>GSHMLEGGVEVLSVVTGEDSITQIELYLNPRMGVNSPDLPTTSNWYTYTYDLQPKGSSPDQPIKENLPAYSVARVSLPMLNEDITCDTLQMWEAISVKTEVVGISSLINVHYWDMKRVHDYGAGIPVSGVNYHMFAIGGEPLDLQGLVLDYQTQYPKTTNGGPITIETVLGRKMTPKNQGLDPQAKAKLDKDGNYPIEVWCPDPSKNENSRYYGSIQTGSQTPTVLQFSNTLTTVLLDENGVGPLCKGDGLFISCADIVGFLFKTSGKMALHGLPRYFNVTLRKRWVKN[20x]

The human Merkel cell polyomavirus (MCPyV or MCV) was discovered in 2008 and found to be clonally integrated into Merkel cell carcinomas (MCCs), establishing it as the first human oncovirus from the polyomavirus family. Polyomavirus infectious entry is initiated by the major capsid protein VP1, which attaches to cellular receptors to promote internalization and transport of the viral genome into the nucleus for replication. MCPyV VP1 is a symmetric ring-shaped homopentamer with the five VP1 monomers arranged around a central five-fold axis. Each monomer is composed of two antiparallel β-sheets, which together form a β-sandwich with jelly-roll topology.

We next determined high-resolution structures of MCPyV VP1 in complex with three different sialylated oligosaccharides derived from the in vitro binding partner GT1b. In each complex, electron density was only observed for the Neu5Ac-α2,3-Gal motif that is common to all three investigated oligosaccharides and is also present in GT1b. This disaccharide motif binds to a shallow binding site on the outer surface of VP1, which is formed entirely by residues of the BC-, DE- and HI-loops of one VP1 monomer. In all instances where ligand was bound, the α2,3-glycosidic linkage between Neu5Ac and Gal adopts the same conformation (torsion angles of −54° and −6°) that is preferred in solution and that is also found in complexes of mPyV VP1, hemagglutinins of influenza A viruses and wheat-germ agglutinin with linear α2,3-sialylated oligosaccharides. Neu5Ac forms the major contact point with MCPyV as it contributes most interactions and is best defined by electron density. Most of its protruding functional groups are engaged by the protein. Its carboxyl group forms a salt bridge and hydrogen bonds with K299 and S297 in the HI-loop and water-mediated hydrogen bonds with D145 and S297. The Neu5Ac N-acetyl group faces away from the fivefold axis, interacting with residues in the BC-loop. It makes hydrophobic interactions with the side chains of W76 and Y81 and hydrogen bonds with D82, which forms a salt bridge with K295. Furthermore, the O4 hydroxyl group of Neu5Ac interacts with Y143 and D145 in the DE-loop via a water molecule. The Gal residue does not contact the protein directly and exhibits elevated temperature factors, but can be docked unambiguously into the electron density.>MSKYKLIMLRHGEGAWNKENRFCSWVDQKLNSEGMEEARNCGKQLKALNFEFDLVFTSVLNRSIHTAWLILEELGQEWVPVESSWRLNERHYGALIGLNREQMALNHGEEQVRLWRRSYNVTPPPIEESHPYYQEIYNDRRYKVCDVPLDQLPRSESLKDVLERLLPYWNERIAPEVLRGKTILISAHGNSSRALLKHLEGISDEDIINITLPTGVPILLELDENLRAVGPHQFLGDQEAIQAAIKKVEDQGKVKQAKKLEHHHHHH[2x]

Bisphosphoglycerate mutase (BPGM) is an erythrocyte-specific multifunctional enzyme that is responsible for the regulation of 2,3-bisphosphoglycerate (2,3-BPG) in red blood cells through its synthase and phosphatase activities; the latter enzymatic function is stimulated by the endogenous activator 2-phosphoglycolate (2-PG). 2,3-BPG is a natural allosteric effector of hemoglobin (Hb) that is responsible for decreasing the affinity of Hb for oxygen to facilitate tissue oxygenation. BPGM is a multifunctional enzyme, functioning as a 2,3-BPG synthase, a 2,3-BPG phosphatase and a phosphoglycerate mutase. The phosphatase activity is responsible for the hydrolysis of 2,3-BPG to 3-phosphoglycerate (3-PGA), an intermediate in the main glycolytic pathway.

The crystal structure of BPGM complexed with 3-PGA and 2-PG has been determined to 2.25 Å resolution. The B factor of 3-PGA in monomer A is 39.0 Å2, that of 2-PG in monomer B is 63.9 Å2 and that of 2-PG in the dimer interface is 56.3 Å2, consistent with the weakest ligand density being observed in monomer B, and likely suggesting different affinities for the ligands at these binding sites. The 3-PGA phosphoryl O atoms interact with the guanidino groups of Arg100 (2.7–2.9 Å), Arg116 (2.7 Å) and Arg117 (2.9 Å), the amide of Asn190 (3.2 Å) and the hydroxyl of Tyr92 (2.6 Å). However, unlike monomer A, a significant portion of the C-terminus of monomer B, which partly forms the active-site structure, was missing (13 residues) due to disorder. Also, unlike monomer A, the side chains of several other amino acids located in the active-site pocket of monomer B, including Arg100, Arg116 and Arg117, were highly disordered, as shown by weak or missing electron density. The phosphate O atoms form direct hydrogen-bond interactions with the imidazole of His65 (3.3 Å) in monomer A and the carboxyl of Glu72 (3.6 Å) in monomer B. In addition, the carboxyl group of 2-PG makes water-mediated interactions with the imidazole group of His65 in monomer B and the carboxyl of Glu72 in monomer A.>MSQDVNELSKQPTPDKAEDNAFFPSPYSLSQYTAPKTDFDGVEHKGAYKDGKWKVLMIAAEERYVLLENGKMFSTGNHPVEMLLPLHHLMEAGFDVDVATLSGYPVKLELWAMPTEDEAVISTYNKLKEKLKQPKKLADVIKNELGPDSDYLSVFIPGGHAAVVGISESEDVQQTLDWALDNDRFIVTLCHGPAALLSAG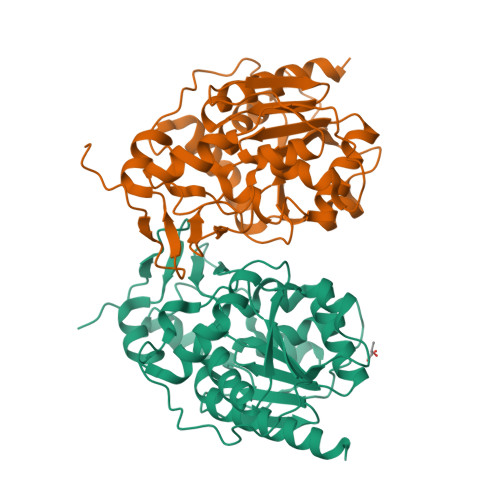LNREKSPLEGYSVCVFPDSLDEGANIEIGYLPGRLKWLVADLLTKQGLKVVNDDMTGRTLKDRKLLTGDSPLASNELGKLAVNEMLNAIQNKLEHHHHHH[8x]> KKVCACPKILKPVCGSDGRTYANSCIARCNGVSIKSEGSCPTG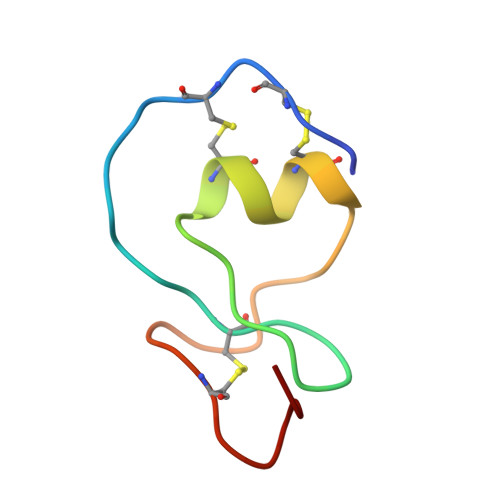ILN>[2x]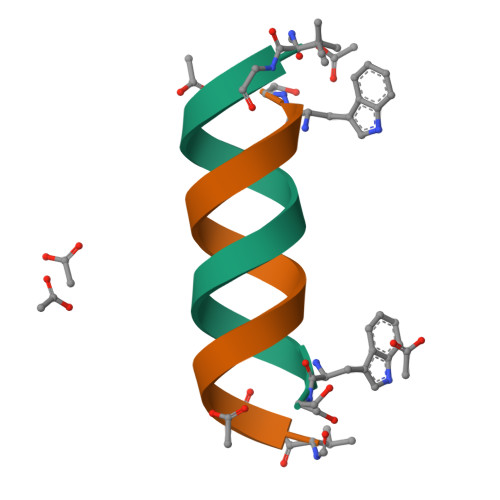VGALAVVVWLWLWLWX>GSGSTLREVARVTNVKDTEVIYFSVGAVLSGYKVIYDKVTQRSYFIPELPTGTTAVSLSSSAILVHSAGSVDLGALAVSREEYVTLSGTFDSGAVINTKNELLTHTDGKYRWDGTLPKTVAAGSTPATTGGVGSGAWLSVGDASLKSNLNKPNGLSYIGTVSSVSELSSIAGLIGDSIILDSYVDGFNLGGGVMVAVNSDTVVDNIVTFQGNGVVWKRKLFNGVADVYEAGYTGTGDLAIFINKINAVGFDCIVPVSGEITTPIIFDIAKGALIGKNKCTLIESASATGDYYLTIVNTDTDYTNRDVINATALMTGVSFVGKGTRKLAIGGSTSGEVSELRISNCGFISTAGIEFLDNAYRILFDKCALSRSFTNSVIFNSPANSGEVIKFNHCWMVDNGGPFTFKNGQFIFDSCSLPAGKKSGYFDPVVALSDNATTVFTNGNIEYQPGQSFVGFTVDGSSRLSISDSTILLPNDYSTVPIVNNGDGVVSLNNCSLPLYGSTTIATGFATRQLIGGLSKKIMSRGCYPRAGFITSNWNLGCIVSPYINSVSNGSGQFENISNWTLSQTGTDVVTVTTGNDVPNDLMFSTSFVLSVPTVGAAANFTQTIIDCEPGRYFQLGFWAKNTTTTLASIRFLDQQGNAVADSIGYNIPVG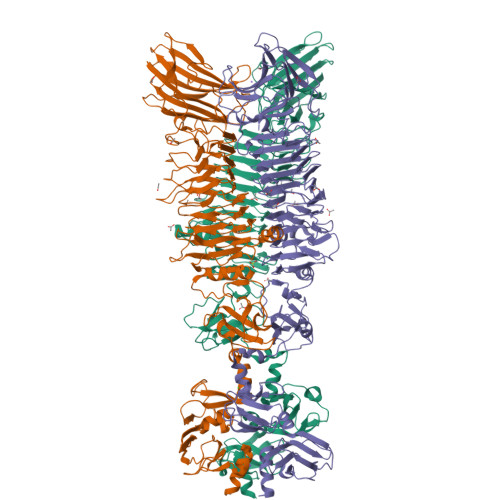NTFNFYALVDCVPPGAYRAEINFNVSSIVGGIAIHNVIYGLI[3x]Glutaryl-CoA dehydrogenase (GCDH) is an acyl-CoA dehydro­genase (ACDH) which catalyzes an intermediate step in the metabolic breakdown of lysine and tryptophan. Unlike other flavoproteins within this family, GCDH (EC 1.3.99.7) performs α,β-dehydrogenation as well as decarboxylation of its sub­strate glutaryl-CoA to yield the product crotonyl-CoA. Transfer of electrons from the glutaryl-CoA precursor to the electron-transfer flavoprotein is mediated by the cofactor flavin adenine dinucleotide (FAD) in both prokaryotic and eukaryotic electron-transport chains. Like other ACDHs, GCDH from B. pseudomallei (BpGCDH) exists as a homotetramer with tetrahedral symmetry and possesses an overall fold similar to that of the human enzyme.

Here, we report the first structures of GCDH from B. pseudomallei (BpGCDH), including the first apo structure of any GCDH characterized in the absence of FAD. Although highly homologous in structure and sequence, the apo structure of GCDH from B. pseudomallei revealed a loss of secondary structure and increased regions of disorder when compared with the previously determined human GCDH ternary complex. In all four protomers of BpGCDH, electron density was too poor to model from Thr139 to Asp145. This loop extends from the pseudo-β-barrel region into part of the FAD-binding site, as seen in Thr136–Asp143 of hGCDH, acting as a wall to separate the diphosphate of FAD from the alkyl pantothenate moiety of glutaryl-CoA. In a different region of the human complex, a short α-helical turn comprises part of the flavin-binding site and the adjacent protomer interface. This helical character is lost in two of the four protomers of the apo BpGCDH structure, further suggesting that FAD binding helps to maintain secondary structure at crucial protomer protein binding surfaces. Side-chain rotamers between the two enzymes also tend to be well conserved along this sequence, with the exception of Tyr373. In our apo BpGCDH structure this tyrosine is flipped nearly 180° from its position in the human complex, with a distance of approximately 9.2 Å between aromatic hydroxyls. In the absence of substrate and cofactor Tyr373 no longer hydrogen bonds to Arg97. Instead, the apo structure reveals Glu370 participating in a water-mediated contact to Arg97, with the catalytic glutamate carboxyl having moved 3.8 Å away from where it sits in the human enzyme. Thus, the tyrosine side chain of apo BpGCDH must rotate by 180° and displace a conserved water molecule in order to attain a conformation suitable for FAD binding.

>SMAAATFHWDDPLLLDQQLADDERMVRDAAHAYAQGKLAPRVTEAFRHETTDAAIFREMGEIGLLGPTIPEQYGGPGLDYVSYGLIAREVERVDSGYRSMMSVQSSLVMVPIFEFGSDAQKEKYLPKLATGEWIGCFGLTEPNHGSDPGSMVTRARKVPGGYSLSGSKMWITNSPIADVFVVWAKLDEDGRDEIRGFILEKGCKGLSAPAIHGKVGLRASITGEIVLDEAFVPEENILPHVKGLRGPFTCLNSARYGIAWGALGAAESCWHIARQYVLDRKQFGRPLAANQLIQKKLADMQTEITLGLQGVLRLGRMKDEGTAAVEITSIMKRNSCGKALDIARLARDMLGGNGISDEFGVARHLVNLEVVNTYEGTHDIHALILGRAQTGIQAFF[4x]The transient receptor potential channel subfamily A member 1 (TRPA1) ion channel is an evolutionary conserved polymodal sensor responding to noxious temperature or chemical stimuli. TRPA1 is a member of the transient receptor potential (TRP) superfamily with a symbolic cytosolic domain formed by a particularly large number of ankyrin repeats (ARs). While the four isoforms exhibit similar responses to electrophilic agonists, they exhibit distinct thermosensitivities, and the dTRPA1-A isoform is shown to be the most heat-sensitive to either absolute temperature or heating rate. As with hTRPA1, the transmembrane domain of each subunit consists of six transmembrane α-helices (S1–S6), with S1–S4 forming the voltage-sensor-like domain (VSLD) and S5–S6 forming the pore domain organised in a domain-swapped manner.

However, in state-1, the ARD is prominently stabilised in a four-leaf propeller-shaped structure, and the high local resolutions allow modelling of 17 ARs in total (AR0–AR16). For state-1, 1053 residues (88.0% of the total number of residues) were structurally built with 953 residues assigned. The N-terminus starts from residue number 58, with most of the ARs faithfully assigned. In state-1, IFH and the succeeding loop (named IFH-loop) insert into a pocket formed by the pre-S1 helix, S1, TRP helix and S4–S5 linker and are stabilised by hydrogen bonding and ionic and hydrophobic interactions with adjacent elements. Compared with the state-2 structure of dTRPA1-A, these interactions and the insertion of the IFH-loop cause pre-S1 to rotate around the pivot at the joint of pre-S1 and S1 by 12˚. Strikingly, compared with that of state-2 structure, the coiled-coil domain has a large downward movement with ~12–13 Å. Besides the coiled-coil domain, two new interfaces are identified between neighbouring subunits in the ARD domain of the state-1 structure. One is between AR16 of one subunit and the nexus domain from the adjacent subunit (the loop between the first two β-strands), named interface-1, and the other is within the ARDs between two adjacent subunits (AR6–AR9 of one subunit and AR12–AR14 of the neighbouring subunit), named interface-2. Missing of the state-1 structure at the high temperature suggests that it might be a resting or pre-sensitised state prior to heat stimuli. The state-1 structure might represent an initial closed, or resting state of dTRPA1-A isoform.

>MTSGDKETPKREDFASALRFLMGGCAREPEMTAMAPLNLPKKWARILRMSSTPKIPIVDYLEAAESGNLDDFKRLFMADNSRIALKDAKGRTAAHQAAARNRVNILRYIRDQNGDFNAKDNAGNTPLHIAVESDAYDALDYLLSIPVDTGVLNEKKQAPVHLATELNKVKSLRVMGQYRNVIDIQQGGEHGRTALHLAAIYDHEECARILITEFDACPRKPCNNGYYPIHEAAKNASSKTMEVFFQWGEQRGCTREEMISFYDSEGNVPLHSAVHGGDIKAVELCLKSGAKISTQQHDLSTPVHLACAQGAIDIVKLMFEMQPMEKRLCLSCTDVQKMTPLHCASMFDHPDIVSYLVAEGADINALDKEHRSPLLLAASRSGWKTVHLLIRLGACISVKDAAARNVLHFVIMNGGRLTDFAEQVANCQTQAQLKLLLNEKDSMGCSPLHYASRDGHIRSLENLIRLGACINLKNNNNESPLHFAARYGRYNTVRQLLDSEKGSFIINESDGAGMTPLHISSQQGHTRVVQLLLNRGALLHRDHTGRNPLQLAAMSGYTETIELLHSVHSHLLDQVDKDGNTALHLATMENKPHAISVLMSMGCKLVYNVLDMSAIDYAIYYKYPEAALAMVTHEERANEVMALRSDKHPCVTLALIASMPKVFEAVQDKCITKANCKKDSKSFYIKYSFAFLQCPFMFAKIDEKTGESITTASPIPLPALNTMVTHGRVELLAHPLSQKYLQMKWNSYGKYFHLANLLIYSIFLVFVTIYSSLMMNNIELKAGDNKTMSQYCNMGWEQLTMNLSQNPSVASQIRLDSCEERINRTTAILFCAVVIVVYILLNSMRELIQIYQQKLHYILETVNLISWVLYISALVMVTPAFQPDGGINTIHYSAASIAVFLSWFRLLLFLQRFDQVGIYVVMFLEILQTLIKVLMVFSILIIAFGLAFYILLSKIIDPQPNHLSFSNIPMSLLRTFSMMLGELDFVGTYVNTYYRDQLKVPMTSFLILSVFMILMPILLMNLLIGLAVGDIESVRRNAQLKRLAMQVVLHTELERKLPHVWLQRVDKMELIEYPNETKCKLGFCDFILRKWFSNPFTEDSSMDVISFDNNDDYINAELERQRRKLRDISRMLEQQHHLVRLIVQKMEIKTEADDVDEGISPNELRSVVGLRSAGGNRWNSPRVRNKLRAALSFNKSM[4x]>[2x]MNRESFAAGERLVSPAYVRQGCEARRSHEHLIRLLLEKGKCPENGWDESTLELFLHELAIMDSNNFLGNCGVGEREGR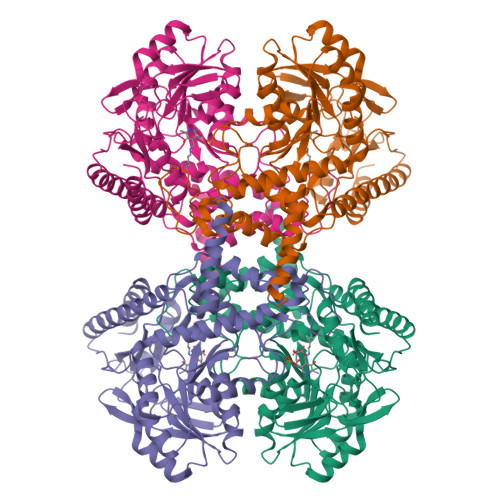VASALVARRHYRFIHGIGRSGDISAVQPKAAGSSLLNKITNSLVLDIIKLAGVHTVANCFVVPMATGMSLTLCFLTLRHKRPKAKYIIWPRIDQKSCFKSMITAGFEPVVIENVLEGDELRTDLKAVEAKVQELGPDCILCIHSTTSCFAPRVPDRLEELAVICANYDIPHIVNNAYGVQSSKCMHLIQQGARVGRIDAFVQSLDKNFMVPVGGAIIAGFNDSFIQEISKMYPGRASASPSLDVLISLLSLGSNGYKKLLKERKEMFSYLSNQIKKLSEAYNERLLHTPHNPISLAMTLKTLDEHRDKAVTQLGSMLFTRQVSGARVVPLGSMQTVSGYTFRGFMSHTNNYPCAYLNAASAIGMKMQDVDLFIKRLDRCLKAVRKERSKESDDNYDKTEDVDIEEMALKLDNVLLDTYQDASS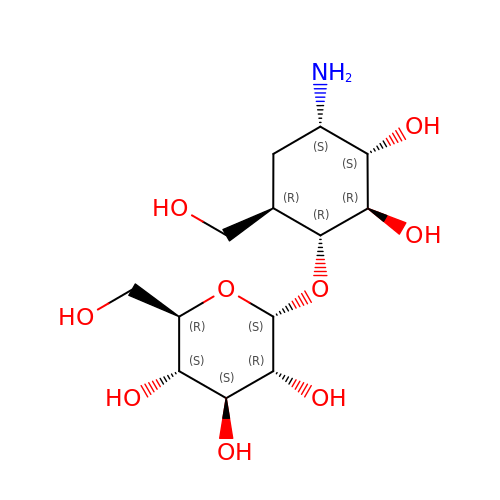(1R,2R,3S,4S,6R)-4-amino-2,3-dihydroxy-6-(hydroxymethyl)cyclohexyl alpha-D-glucopyranoside | C13 H25 N O9 | IURYEWAUXBUYIM-BTADNHFESA-N> MVIVPEGTQLDEKQHIVINNGAEPQSFDPHKTEGVPESNVAYQLLEGLVTSDSEGKLQPGAAESWENTPDFKTWTFHLRKDAKWSNGDPVTAHDFVFAWRRLVDPATAAPYASYLSYLQVENAQDIIDGKKKPAELGVEAKDDYTFVVHATNPVPYAVSLTTHQSLLPLPQKVVEKLGDAWVKKENYVGNGAYKLANHIINEKIEFERNPLYWNDKETVINSATFLAIENPSTDVARYRAGDLDMTSYGLPPEQFAKLKKELLGEVYVTRTLGTYSYELNNKKAPFDNVNIRKALNLSLDRNVITDKVLGQGQTPTYVFTPTYIEEGHLIQQPAYSKEPMAQRNEEAIKLLEEAGYSKANPLKFSILYNTNENHKKVAIAAASMWKANTKGLIDVKLENQEWKTYIDSRRAGRYDVARAGWHADYNQATTFGNYFLSNSSNNTAKYANPEYDKAMAESYAATDAEGRAKAYAKAEEILGKDY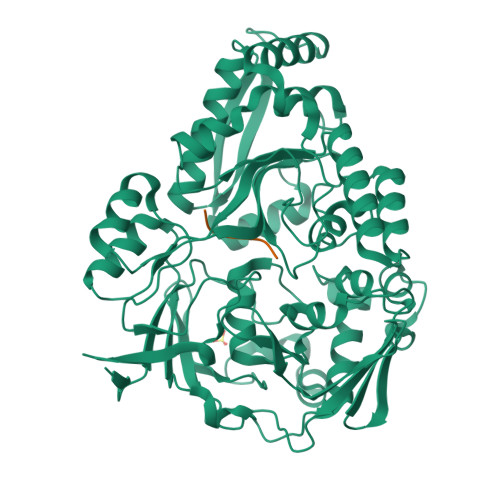GIVPIFNYVNPRLVKPYVKGYSGKDPQDHIYLRNLYIIKHLEHHHHHH;> GIINTL>[2x]MKHHHHHHPMVKEYKTITQIAGPLIFVEKTEPVGYNEIVNIKMGDGTVRRGQVLDSSADIVVVQVFEGTGGLDKDCGVIFTGETLKLPASVDLLGRILSGSG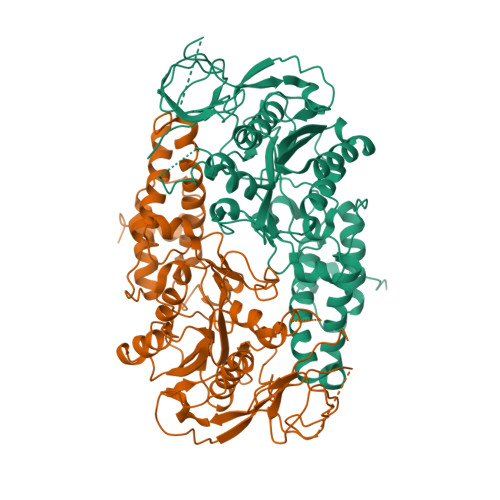EPRDGGPRIVPDQLLDINGAAMNPYARLPPKDFIQTGISTIDGTNTLVRGQKLPIFSASGLPHNEIALQIARQASVPGSESAFAVVFAAMGITNEEAQYFMSDFEKTGALERAVVFLNLADDPAVERIVTPRMALTAAEYLAYEHGMHVLVILTDITNYAEALRQMGAARNEVPGRRGYPGYMYTDLATLYERAGIVKGAKGSVTQIPILSMPGDDITHPIPDLSGYITEGQIVVARELHRKGIYPPINVLPSLSRLMNSGIGAGKTREDHKAVSDQMYAGYAEGRDLRGLVAIVGKEALSERDTKFLEFADLFEDKFVRQGWNENRTIEDTLEIGWQILTHLPENQLGRIDNKYIQKYHPAHRKAK> MSKDVIEYSKLFAKLVNTNDDTKLDDTIASFLYYMFPRELFIRAISLLESSDMFIYILDRVHNKEGNEHTSLIDVLVDEFYKGSSNSLLEYRLIVKDTNDGAPPILVDIAHW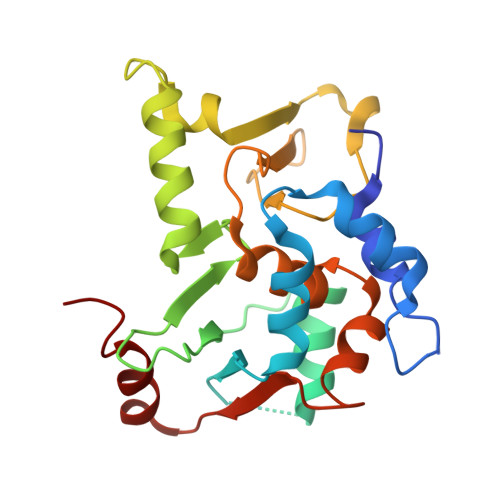FCSCEEFCKYFHEALEKTDEKEELHDVLINEVDDHLQFSDDRFAQLDPHSLSKQWYFKFDKVCCSHLLAFSILLRSSINVLKFFTVNSNKVFVIAIDNIDEWLNLHINIVE>[2x]MHHHHHHGGGGGMNRLAKILP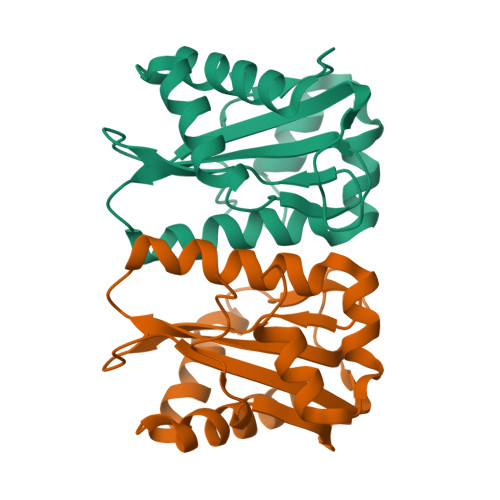LENVVIDLSVTSKKRVFEQAGLIFENQNGIARSTVTDNLFARERLGSTGLGEGVAIPHGRIKGLKHPLAAFVRLAEPIPFEAPDGQPVSLLIFLLVPEQATQAHLEILSEIAQLLSDRDTRERLHTEPDRDELHRLLTQWQP>MGSSHHHHHHSSGLVPRGSLHMSPRVGVTLSGRYRLQRLIATGGMGQVWEAVDNRLGRRVAVKVLKSEFSSDPEFIERFRAEARTTAMLNHPGIASVHDYGESQMNGEGRTAYLVMELVNGEPLNSVLKRTGRLSLRHALDMLEQTGRALQIAHAAGLVHRDVKPGNILIT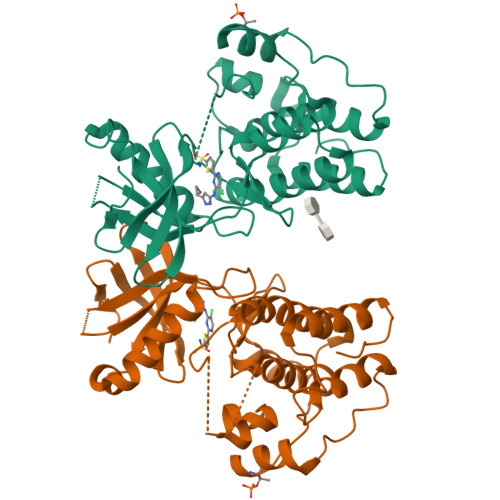PTGQVKITDFGIAKAVDAAPVTQTGMVMGTAQYIAPEQALGHDASPASDVYSLGVVGYEAVSGKRPFAGDGALTVAMKHIKEPPPPLPPDLPPNVRELIEITLVKNPAMRYRSGGPFADAVAAVRAGRRPPRPSQTPPPGRAAPAA[4x]> MKKPVKSWLIASTVAALLAVPAVSQANSEVEKLTKNPANWATWGGNYHGTRYSELKQINTSNVKNLQPAWTFSTGVLRGHEGGPLVVNDVMYIHTP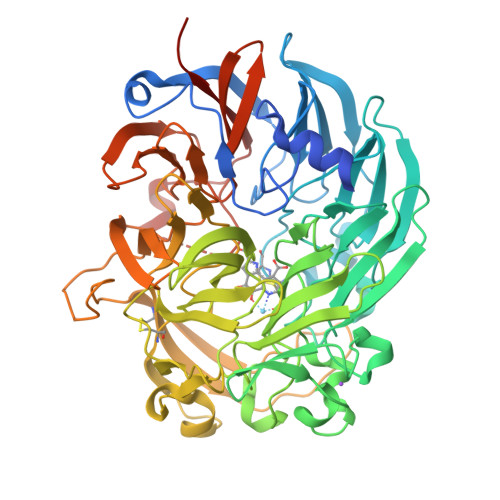FPNTVYAIDQKTQAVIWEYTPQQDADVTIPVMCCDTVNRGLAYGDGKIFLQQSDTVLTALDAKTGKRVWSVQNGDPKLGMTNTQAPLVVKDKVITGISGGEFGVRGFLAAYNIRTGELDWKGYSMGPDADTLINPTKTTTWKDGKVQPVGKDSSTSTWEGDQWKIGGGTTWGWYSYDPELNLVYYGSGNPSTWNPAQRPGDNKWSMSLWARNADTGEVKWVYQMTPHDEWDYDGINEVALVDQEIKGQMRKTAVHFDRNGFGYTLDRVTGELLVAEKFDKAVNWASHVDMKSGRPQVVSQYSTEYNGEDVNTEGVCPAALGSKNQQPVSYSPQTGYFYISGNHVCMDYEPFEVEYTAGQPYVGATLSMFPAGKDVITGKEDGSNNLGQFTAWDATTGKIIWSNKEQFSVWSGSLATAGGVVFYGTLEGYLKAVDAKTGKELYRFKTPSGIIGNVNTWEYEGKQYVGVLSGVGGWAGIGIAAGLDSGEESSNSEGLGAVGAYRSLSSYTKLGGTLTVFALPN> MTIHSCLARRAVSVAASGARAFASGLGARAVAVGALQSARLLHTSSLRAAGAKISPSEMSRLLEERIAGWKTQTSTEEVGRVVSVGDGIARLFGLEGVQAGELVEFQNGMTGMALNLETDNVGVVIFGDDRSVLEGDSVKRTGRIVDVPIGPGLLGRVVDALGNPIDGKGPIPAKERRRVELKAPGIIPRKSVHEPMMTGLKCVDALVPVGRGQRELIIGDRQTGKTAVAVDA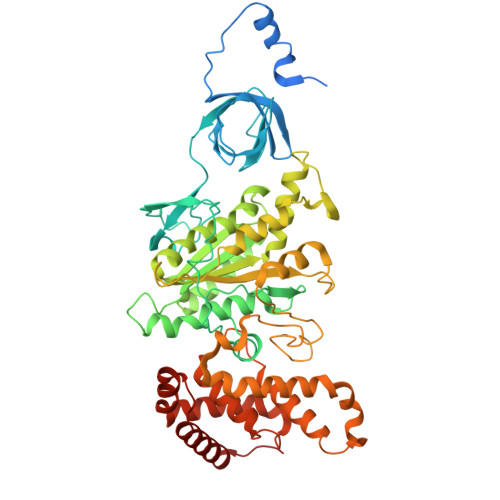IINQKEINDSTDDESKKLYCIYVAVGQKRSTVAQIVKALEQRDAMKYTTVVAATASEAAPLQFLAPYSGCAMGEWFRDSGRHCVIIYDDLSKQATAYRQMSLLLRRPPGREAYPGDVFYLHSRLLERAAKMGDKSGGGSLTALPVIETQAGDVSAYIPTNVISITDGQIFLETELFYKGIRPAINVGLSVSRVGSAAQVKAMKQVAGTMKLELAQYREVAAFAQFGSDLDASTRQLLTRGTALTELLKQRQYSPMKNSVQVCVLYCGVKGYLDPLDPKEISRFESLFIDYINANHQDILKTIETEKELSEKTEAKLRAAVDEFVAMNEFKKK> GPLGSEAQSEKEEAPKPLHKVVVCVSKKLSKKQSELNGIAASLGADYRWSFDETVTHFIYQGRPNDTNREYKSVKERG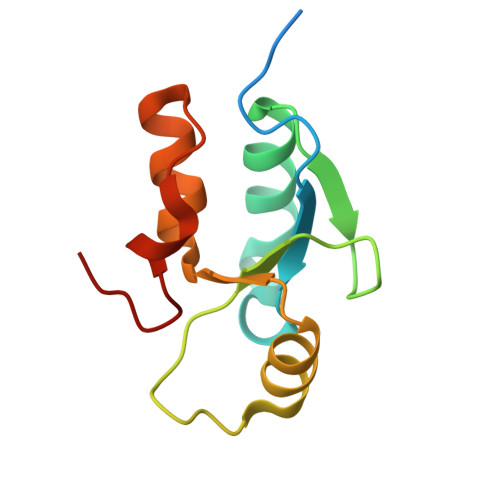VHIVSEHWLLDCAQECKHLPESLYPHTYNPK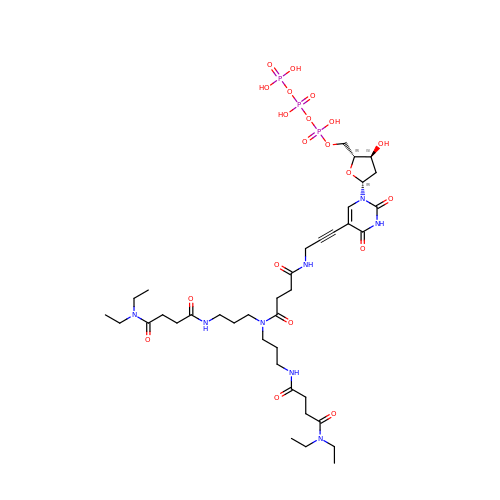2'-deoxy-5-[9-(3-{[4-(diethylamino)-4-oxobutanoyl]amino}propyl)-18-ethyl-5,8,14,17-tetraoxo-4,9,13,18-tetraazaicos-1-yn-1-yl]uridine 5'-(tetrahydrogen triphosphate) | C38 H63 N8 O20 P3 | FRKZJUQJYOJKOB-CMUUVTEDSA-N> NGYENPTY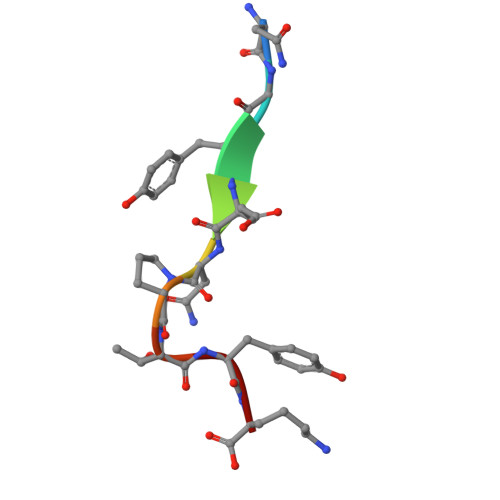K> GSPGISGGGGGIPSGRGELLVSLCYQSTTNTLTVVVLKARHLPKSDVSGLSDPYVKVNLYHAKKRISKKK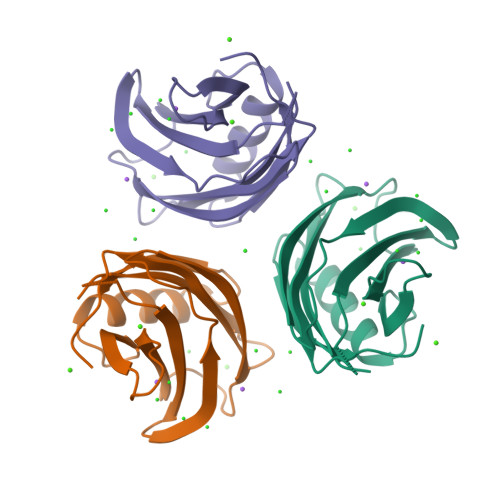THVKKCTPNAVFNELFVFDIPCESLEEISVEFLVLDSERGSRNEVIGRLVLGATAEGSGGGHWKEICDFPRRQIAKWHMLCDG(2S)-2-azanyl-6-[(2-azidophenyl)methoxycarbonylamino]hexanoic acid | C14 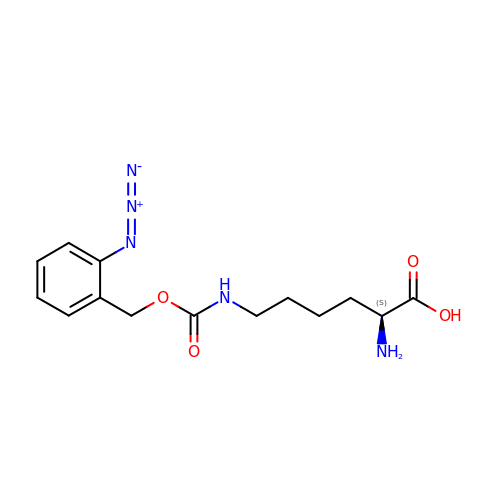H19 N5 O4 | PGNICAOCNIVZRV-NSHDSACASA-N>MVRTTKTSMAAASTVAPEVAMDEGSPSTSQAQVELPRNLEVFNEACGHVFGSSFNREDNSVISDAAAFLFKMHTHSLDGQEAKVLRASEKKRERENAKKSRKAPEAGMRVGRSLILTSRWTEYCATCVPALGSKMKVIKASGDAAMIQMMKDHNSLLRVCVRIEVWKARYVSLVALDERIQTLEDAQWFPYLSGDSYRACPGLVGGYFAKKAAAGERGKNYKKLNQTAIIPPPRFLIIGHRLQIGDQVTLRELLASIAWGLCDGVLAECWSPSQGDGSIGVVVGLPLQATGSCFLVVASHGLSAIADSRIEGTGNTNLLEECIAIQKQDGVIKCKRSGKSLYHCLKETAGAVGR[3x]

The viral nucleoprotein (NP), a key component of the replication machinery, packages the viral genome into protective ribonucleoprotein particles. Although TiLV-NP is considerably smaller than its influenza counterpart and unrelated in sequence, it maintains the same topology and domain organisation. This comprises a head and body domain between which is a positively charged groove, where single-stranded RNA binds. In addition, an oligomerisation loop inserts into a hydrophobic pocket in the neighbouring NP, the flexible hinges of which allow variable orientation of adjacent NPs.

Model building of the nearly full-length TiLV-NP (lacking the first 33 residues) and associated RNA (deposited with generic purine or pyrimidine bases) was performed de novo in COOT using the map corresponding to two RNA-bound NPs extracted from the TiLV-NP pseudo-C5 pentamer, at 2.9 Å resolution. Importantly, both the quality of the RNA density in the 2.9 Å resolution focused map of covering two adjacent NPs from the pseudo-C5 oligomer and the A-from double-stranded RNA helix in the pseudo-C2 oligomer unambiguously reveal the 5′ to 3′ RNA directionality of the RNA bound to TiLV-NP. As mentioned, in the 2.9 Å resolution structure derived from the focused map of two NPs from the pseudo-C5 oligomer, a total of 12 nucleotides are modelled within one NP. Starting from the 5′ to the 3′ end, the G1 phosphate is stabilised by N225 from the head domain, with its base nestled in a pocket formed by I229, R241, and L285 of the body domain. Weaker density is observed from C2 to A4 as they are not directly stabilised by TiLV-NP but rather stack with each other until reaching U8. A5 and A6 phosphates interact with a triplet of positively charged residues K151, K136, and K139, while A7 ribose O2′ is stabilised by hydrogen bonding with R198 from the head domain. The phosphate group of U8 interacts with K134, and its base is stabilised by N154. U9 takes a sharp turn, repelled by R198, with its base sandwiched between L131, L85 and K83. U10 and A11 phosphates are stabilised by K91, while U10 base is wedged between R198 and F208, which stacks with Y207 to further stabilise A11 base. Finally, U12 phosphate group is surrounded by positively charged residues (R94, K90), while its base stacks with A11.> GPDPSIFSPKPEILFSSWDHLEISTHLIRLSEKHSDLFVPSLYTPSTCFSIERAVLKDLHLYDSSTQSVLDHPDSTQCHHQNNYQDYPHLADRDCQNFRIYAYPLWHHPSAHNPEEMNSMMLSTARRGFAGISHWTLVIVNLDRREVVFFDSLAN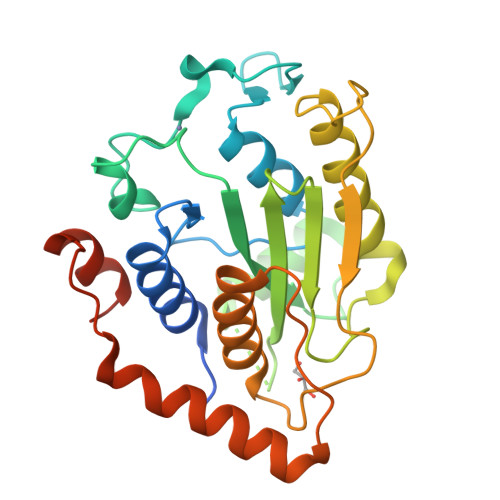FINNRLIDPALNSIATRLGNVYPDANGALSPFIVKKVIKTPIQQDSTSCGIWLSLFLDKYLDNPDYVPPLMGGRQAQYFLQEFLETIPQRPITQASDCTLNVLGITCDQVENSSNML N-[2-(2-hydroxyethyl)-3-{5-[(5-methyl-4,5,6,7-tetrahydropyrazolo[1,5-a]pyrazin-2-yl)amino]-6-oxo-1,6-dihydropyridazin-3-yl}phenyl]-1-benzothiophene-2-carboxamide 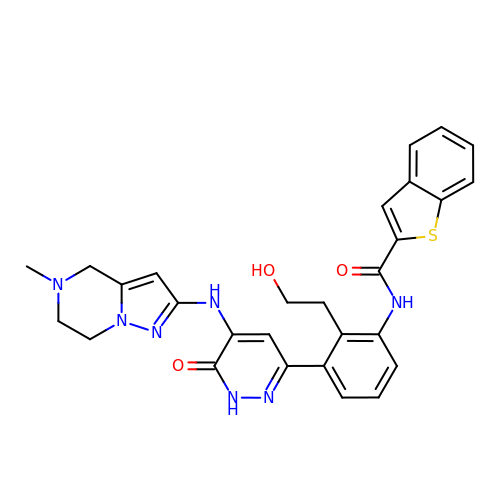| C28 H27 N7 O3 S | MFRXRCVCUQSDMP-UHFFFAOYSA-N> ARPTFHITVGDPHKVGDLATSHIVYSVRTKTTSKAYKQPEFEVKRRYRDFLWLYNTLH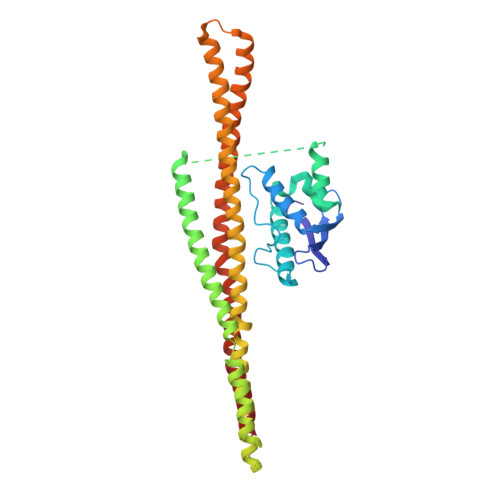SNNPGVVVPPPPEKQAVGRFESNFVESRRAALEKMLNKIAAHPTLQLDADLKLFLESESFNIDVKHKERKEPPLGESKGVFGSLGFGGGGNKFVEQDDWFHDRRVYLDALENQLKALLKAMDNMVAQRKAMAEAAADFSASLHALSTVELSPTLSGPLDALSELQLAIRDVYERQAQQDVLTFGIIIEEYIRLIGSVKQAFSQRQKAFHSWHSAESELMKKKAAQDKLLRQGKTQQDRLNQVNAEVIDAERKVHQARLLFEDMGRLLRSELDRFEREKVEDFKSGVETFLESAVEAQKELIEKWETFLMQ> MAGPVKDREAFQRLNFLYQAAHCVLAQDPENQALARFYCYTERTIAKRLVLRRDPSVKRTLCRGCSSLLVPGLTCTQRQRRCRGQRWTVQTCLTCQRSQRFLNDPGHLLWGDRPEAQLGSQADSKPLQPLPNTAHSISDRLPEEKMQT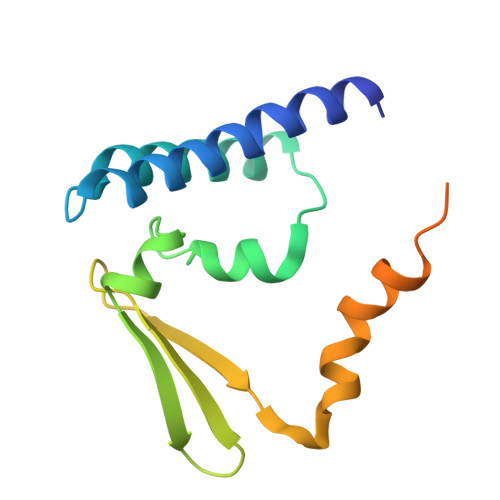QGSSNQ>SVERIYQKKTQLEHILLRPDTYIGSVELVTQQMWVYDEDVGINYREVTFVPGLYKIFDEILVNAADNKQRDPKMSCIRVTIDPENNLISIWNNGKGIPVVEHKVEKMYVPALIFGQLLTSSNYDDDEKKVTGGRNGYGAKLCNIFSTKFTVETASREYKKMFKQTWMDNMGRAGEMELKPFNGEDYTCITFQPDLSKFKMQSLDKDIVALMVRRAYDIAGSTKDVKVFLNGNKLPVKGFRSYVDMYLKDKLDETGNSLKVIHEQVNHRWEVCLTMSEKGFQQISFVNSIATSKGGRHVDYVADQIVTKLVDVVKKKNK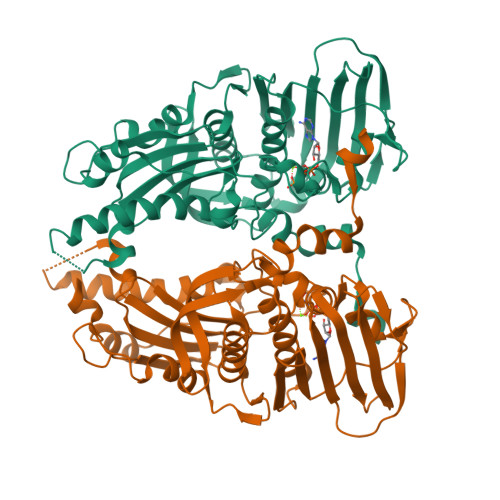GGVAVKAHQVKNHMWIFVNALIENPTFDSQTKENMTLQPKSFGSTCQLSEKFIKAAIGCGIVESILNWVKFKAQVQLNKKCS[2x]> MTPDIILQRTGIDVRAVEQGDDAWHKLRLGVITASEVHNVIAKPRSGKKWPDMKMSYFHTLLAEVCTGVAPEVNAKALAWGKQYENDARTLFEFTSGVNVTESPIIYRDESMRTACSPDGLCSDGNGLELKCPFTSRDFMKFRLGGFEAIKSAYMAQVQYSMWVTRKNAWYFANYDPRMKREGLHYVVIERDEKYMASFDEIVPEFIEKMDEALAE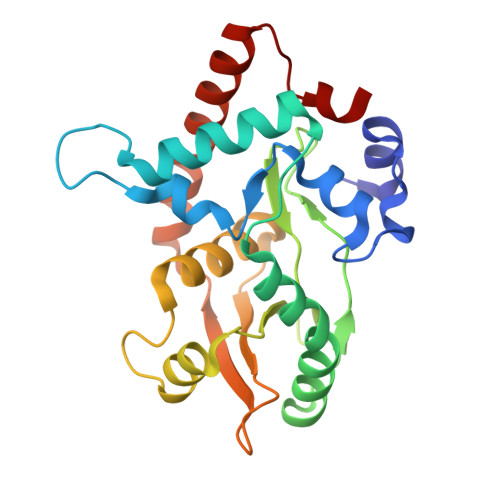IGFVFGEQWR LIN-41 belongs to the TRIM-NHL protein family. These proteins contain a TRIpartite Motif (TRIM) consisting of a RING finger domain (commonly endowing a protein with E3 ubiquitin ligase activity, for example), two B-Box motifs and a coiled-coil domain. Additionally, they also carry six so-called NHL repeats (named after NCL-1, HT2A and LIN-41) and may contain a filamin domain, which have been implicated in both protein-protein and protein-RNA interactions. To understand how this reprogramming is controlled, we searched for C. elegans mutants in which the activation of embryonic genome, a landmark event demarcating the switch from a germline- to embryo-specific transcription, is initiated precociously in germ cells. This screen identified a novel function for LIN-41, a member of the TRIM-NHL protein family, in preventing a premature onset of embryonic-like differentiation and teratoma formation in developing oocytes, thus ensuring a successful passage between generations.

One previously isolated lin-41 allele, ma104, is a transposon insertion into the sequence coding for the filamin domain. We found that the ma104 mutation resulted in an insertion of 16 amino acids into the filamin domain. To gain a mechanistic insight into the ma104 mutation, the filamin domain (residues 691–821) was subcloned, overexpressed in bacteria, and the protein purified to homogeneity. The protein was crystallized and the structure determined at high resolution (1.68 Å; for data collection and refinement statistics, see Table S1). The final crystallographic model encompasses residues 691–729 and 758–820, whereas a long insert (730–757) that is only found in Caenorhabditis LIN-41 protein sequences could not be built due to high flexibility. We found that the LIN-41 filamin structure exhibits a classical immunoglobulin (IG)-like domain fold consisting of seven β-strands arranged in two antiparallel β-sheets. Importantly, the 16-residue insertion present in the ma104 allele maps to the mid-section of the second β-strand and is very likely perturbing the filamin IG-like fold. Specifically, the 16-residue insert will prevent completion of one of the β-sheets resulting in solvent access to the hydrophobic protein core of the IG-like β-sandwich and thereby severely destabilizing the fold. This makes it very unlikely that the filamin domain of the ma104 allele is properly folded to exert its biological function.

> GPSGPCAKNSSIVGDSFKKAIRERQTVIYVQLRDACGDLLSSSIAATQPTSQALLPHQEPHSHLEQAMPTSDVQAFVISPDGSTVEVTMTPRENGIVALSYYPSIEGSYTLNILVKGTPISGCPTTMDIRRGR> GKILLLGPERKWLRDFLESFEDEVTQYQD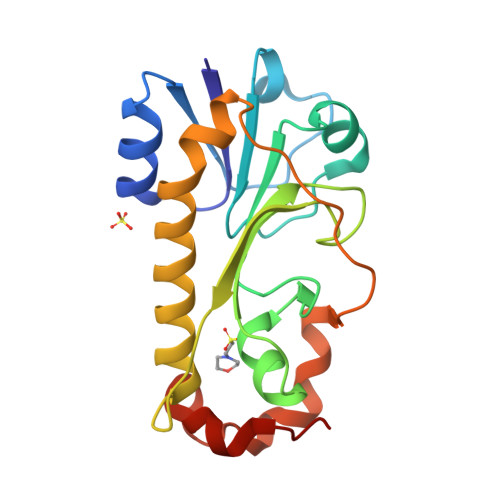KLDKKSAILNNVDFIISYGYRYIIHPDIVERFKQRAINLHISYLPWNKGADPNLWSFLEDSPKGVTIHYIDSGLDTGEIIVQREVTYYENDTLRTTYERLTQTIEKLFMEYWPLIRLGKIRGIPQPKGGSYHKLKDKEKYLYLLTDGWDTPVQKLIGKAQNNE>[4x]GPSGGEVALEHKKKIQKQ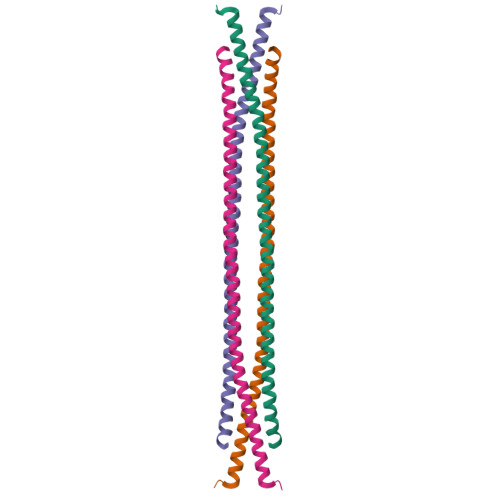LEHLKKLRKSGEEQRSYGEEKAVSFLKQTEALKQRVQRKLEQVYYFLEQQEHFFVASLEDVGQMVGQIRKAYDTRVSQDIALLDALIGELEAKE>TREARISRAKRAFVSTPSVRKILSYMDRCRDLSDLESEPTCMMVYGASGVGKTTVIKKYLN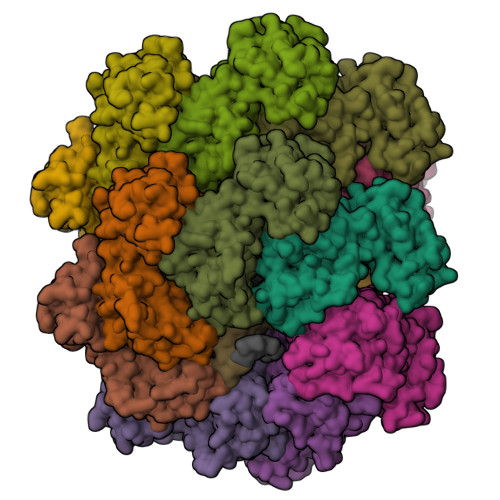QAAAAAAAGGDIIPVLHIELPDNAKPVDAARELLVEMGDPLALYETDLARLTKRLTELIPAVGVKLIIIDEFQHLVEERSNRVLTQVGNWLKMILNKTKCPIVIFGMPYSKVVLQANSQLHGRFSIQVELRPFSYQGGRGVFKTFLEYLDKALPFEKQAGLANESLQKKLYAFSQGNMRSLRNLIYQASIEAIDNQHETITEEDFVFASKLTSGDKPNSWKNPFEEGVEVTEDMLRPPPKDIGWEDYLRH[14x]Heterotrophic bacteria utilize GG phosphorylase (GGP), a member of the GH13_18 family, via a two-step process consisting of phosphorolysis and hydrolysis for GG catabolism. Like MaGGP, MsGGP falls in the GH13_18 subfamily. The crystal structure of MsGGP, akin to other proteins in the GH13_18 family, consists of four domains: A (residues 1–85, 165–290, and 347–429), B (residues 86–164), B' (residues 291–346), and C (residues 430–480). The proposed reaction mechanism for the GH13_18 family involves a double displacement reaction, forming a covalent enzyme–glucosyl intermediate.

To the best of our knowledge, this represents the inaugural structure of a phosphorylase complex containing αGlc1-P within the GH13_18 subfamily. The MsGGP–αGlc1-P crystal (P212121 space group) contains six protomers (chains A, B, C, D, E, and F) in the asymmetric unit. In the asymmetric unit of the MsGGP–αGlc1-P structure, two protomers are characterized by the presence of a glucose and a glycerol molecule occupying the active site (subunits B and F), whereas two other protomers showcase an αGlc1-P molecule in the active site (subunits A and E) with clearly defined electron density. Notably, two additional protomers in the unit (subunits C and D) do not exhibit any ligand binding in the active region. The αGlc1-P could be modeled in density but appears slightly crowded because of the narrow binding pocket of MsGGP, suggesting a high degree of substrate selectivity. Because of steric hindrance, the phosphate group is oriented downward, resulting in a displacement of approximately 1.6 Å from the anomeric carbon compared with its position in the MsGGP–Glc–Gol structure. The glucosyl moiety of αGlc1-P is stabilized by hydrogen bonds through direct interactions with residues Asp49, His87, Arg188, Asp190, Glu231, His288, Asp289, and Arg390, which align with the glucose in the MsGGP–Glc–Gol structure. The phosphate group of αGlc1-P is effectively stabilized, oriented toward the exit channel, forming two hydrogen bonds and three salt bridges with Tyr335, Gln336, Arg131, His233, and Arg390. Conversely, in the MsGGP–αGlc1-P complex structure, loop A undergoes a conformational change, approaching loop B. Despite pushing loop B toward the active center, the channel formed by these two loops measures less than 5 Å. In contrast, in the MsGGP–αGlc1-P complex, the structure remains in a closed state to promote αGlc1-P hydrolysis.

>[6x]MLLKNAVQLICYPDRIGNNLTDLHTAVEKHLSDAIGGLHILPFFPSNADGGFSPLTHKEVDPAFGTWDDIEAFTGKYDLCVDLTVNHISDESPEFRDFIANGFDSEYADLFVHVDRFGDISPDDMAKIHIRKEKEPFREVTLADGTKTRVWCTFTEQQIDLNYDGDLAYRLMESYIGFLTSKGVNLLRLDAFGYTTKRIGTSCFLVEPEVYRILDWINEVAFKHGAECLPEVHDHTSYQYAISRRNMHPYGFALPPLLLYSLLDANSVYLKNWLRMCPRNMVTVLDTHDGICIPDVEGVLPDDKIKVLIDNIDARSADPIMRRSAANIHSVGAIYQLTCTFYDALMQNDDAYIAARAIQFFTPGIPQVYYVGLLAGCNDQELMEKTGELRDINRNYYTLNEMDEAMEKPVVQRLLTLMKFRTNYPAFDGHFELNYSNDSSVAMAWRHGEHYCHLFVDLNFNTSKIQYVDVKSGETRDLEF(2E)-N-hydroxy-3-{1-[2-(1H-indol-3-yl)ethyl]piperidin-4-yl}prop-2-enamide | C18 H23 N3 O2 | 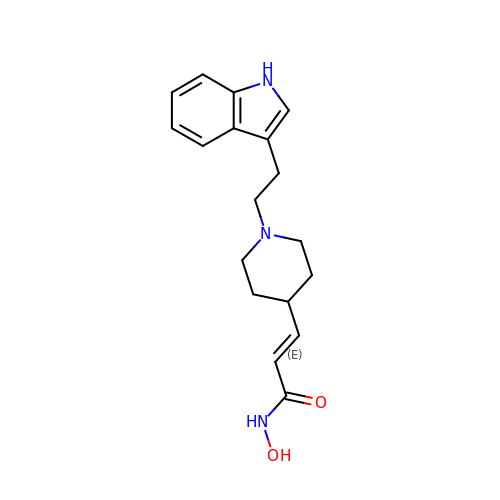ULPMTANVOCUWOD-AATRIKPKSA-N ALPHA-METHYL-L-GLUTAMIC ACID | C6 H11 N O4 | 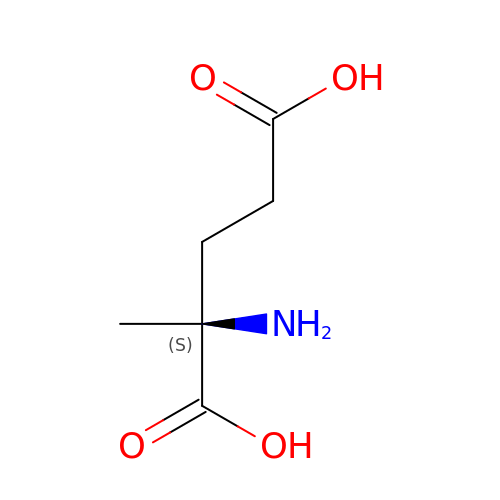QHSCIWIRXWFIGH-LURJTMIESA-N> MSNT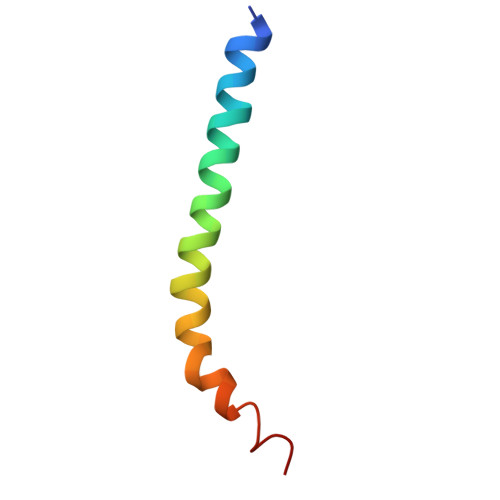CDEKTQSLGVKFLDEYQSKVKRQIFSGYQSDIDTHNRIKDEL>[2x]MVDGNYSVASNVMVPMRDGVRLAVDLYRPDADGPVPVLLVRNPYDKFDVFAWSTQSTNWLEFVRDGYAVVIQDTRGLFASEGEFVPHVDDEADAEDTLSWILEQAWCDGNVGMFGVSYLGVTQWQAAVSGVGGLKAIAPSMASADLYRAPWYGPGGALSVEALLGWSALIGTGLITSRSDARPEDAADFVQLAAILNDVAGAASVTPLAEQPLLGRLIPWVIDQVVDHPDNDESWQSISLFERLGGLATPALITAGWYDGFVGESLRTFVAVKDNADARLVVGPWSHSNLTGRNADRKFGIAATYPIQEATTMHKAFFDRHLRGETDALAGVPKVRLFVMGIDEWRDETDWPLPDTAYTPFYLGGSGAANTSTGGGTLSTSISGTESADTYLYDPADPVPSLGGTLLFHNGDNGPADQRPIHDRDDVLCYSTEVLTDPVEVTGTVSARLFVSSSAVD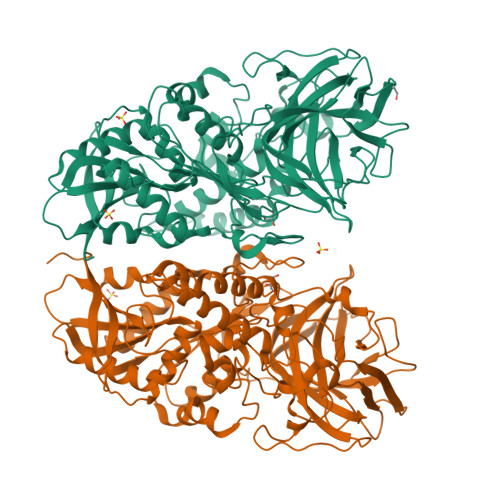TDFTAKLVDVFPDGRAIALCDGIVRMRYRETLVNPTLIEAGEIYEVAIDMLATSNVFLPGHRIMVQVSSSNFPKYDRNSNTGGVIAREQLEEMCTAVNRIHRGPEHPSHIVLPIIKRKLAAALEHHHHHH> MSHHHHHHSMVD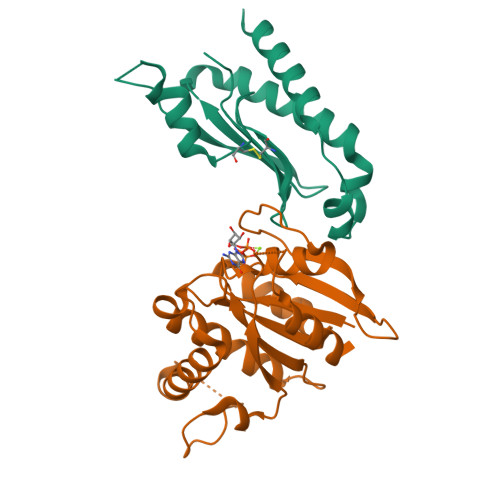FFTIFSKGGLVLWCFQGVSDSCTGPVNALIRSVLLQERGGNNSFTHEALTLKYKLDNQFELVFVVGFQKILTLTYVDKLIDDVHRLFRDKYRTEIQQQSALSLLNGTFDFQNDFLRLLREAEESSKIRAPTTMKKFEDSEKAKKPVRSMIETRGEKPKEKAKNSKKKGAKKEG;> MARKSSQRAVLFVGLCDSGKTLLFVRLLTGQYRDTQTSITDSSAIYKVNNNRGNSLTLIDLPGHESLRFQLLDRFKSSARAVVFVVDSAAFQREVKDVAEFLYQVLIDSMALKNSPSLLIACNKQDIAMAKSAKLIQQQLEKELNTLRVTRSAAPSTLDSSSTAPAQLGKKGKEFEFSQLPLKVEFLECSAKGGRGDTGSADIQDLEKWLAKIA>[3x]MERIDSHVSPRYAQIPTFMRLPHDPQPRGYDVVVIGA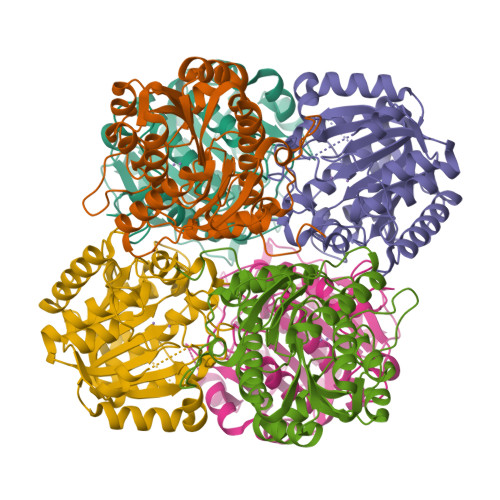PYDGGTSYRPGARFGPQAIRSESGLIHGVGIDRGPGTFDLINCVDAGDINLTPFDMNIAIDTAQSHLSGLLKANAAFLMIGGDHSLTVAALRAVAEQHGPLAVVHLDAHSDTNPAFYGGRYHHGTPFRHGIDEKLIDPAAMVQIGIRGHNPKPDSLDYARGHGVRVVTADEFGELGVGGTADLIREKVGQRPVYVSVDIDVVDPAFAPGTGTPAPGGLLSREVLALLRCVGDLKPVGFDVMEVSPLYDHGGITSILATEIGAELLYQYARAHRTQL>[2x]SNEKIRSQSVLNTLETFFIKENHYDMQREESSIVNACLRYLGYSKSMCHEKMPIFMDIAFIEYCFNLSLDPSSFQNLPITQTQPD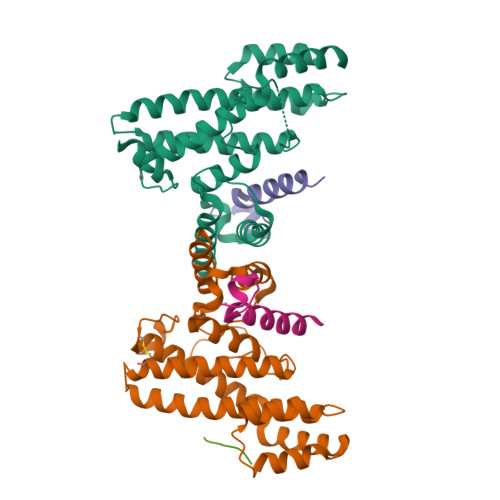SQQILWEYSLISNALERLENIELERQNCMREDGLVKYTNELLLNKETLNNEALKLYSCAKAGICRWMAFHFLEQEPIDHINFTKFLQDWGSHNEKEMEALQRLSKHKIRKRLIYVSQHKKKMPWSKFNSVLSRYIQCTKLQLEVFCDYDFKQREIVKMLTSNIN;>SEACEMCRLGLPHGSFFELLRDWKKIEEFRNKS[2x];> SDNIFVKPGEDLEIPLLSDYSDSENISEKS2-AMINO-1,3-PROPANEDIOL | C3 H9 N O2 | 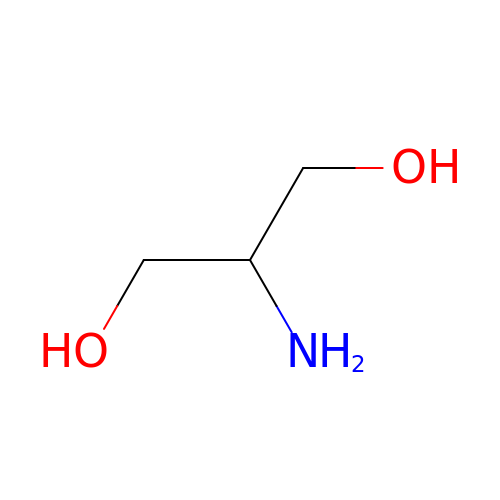KJJPLEZQSCZCKE-UHFFFAOYSA-N> MREILSIHVGQCGNQIADSFWRLALREHGLTEAGTLK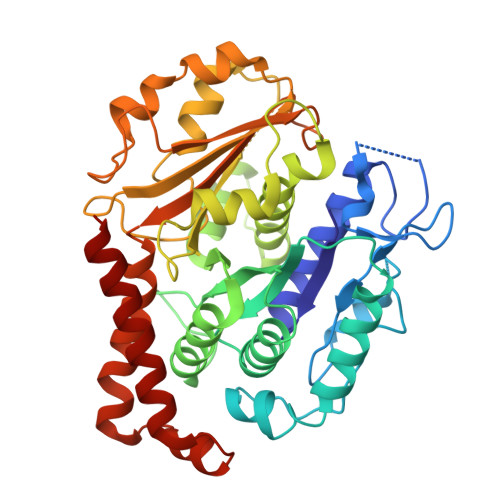EGSNAAANSNMEVFFHKVRDGKYVPRAVLVDLEPGVIARIEGGDMSQLFDESSIVRKIPGAANNWARGYNVEGEKVIDQIMNVIDSAVEKTKGLQGFLMTHSIGGGSGSGLGSLILERLRQAYPKKRIFTFSVVPSPLISDSAVEPYNAILTLQRILDNADGAVLLDNEALFRIAKAKLNRSPNYMDLNNIIALIVSSVTASLRFPGKLNTDLSEFVTNLVPFPGNHFLTASFAPMRGAGQEGQVRTNFPDLARETFAQDNFTAAIDWQQGVYLAASALFRGDVKAKDVDENMATIRKSLNYASYMPASGGLKLGYAETAPEGFASSGLALVNHTGIAAVFERLIAQFDIMFDNHAYTHWYENAGVSRDMMAKARNQIATLAQSYRDAS>DPAVTYYRLEEVAKRNTAEETWMVIHGRVYDITRFLSEHPGGEEVLLEQAGADATESFEDVGHSPDAREMLKQYYIGDVHPNDL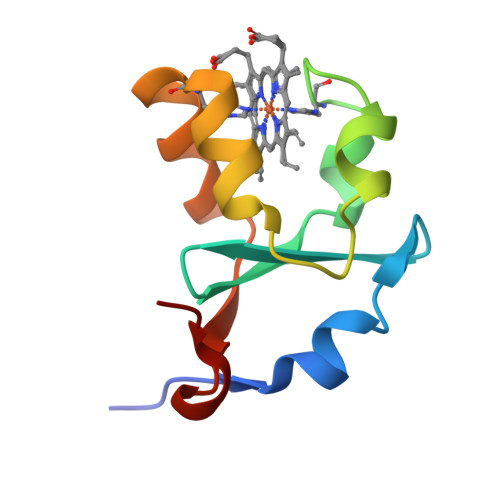KPA[2x]>MGSKLINVEGGNNQDDNKYNSNNVISINNKVNKNDYFIETNKELKINLNFQNNNIISNIFSNINIYDKISNIFINNKKTYMLKYNNNINEENFFISYFEKKDDNFVPISPWHHIDLKNDDGTYNMIVEITKYNYIKLEIQLREKFNVIKQDKKKGKLRYYHNSIYWNYGALPQTYEYPKHIYQNKSKKNKEALLFTGDNDPLDILDIGSACLKIGQVVPVKILGAFTLIDEGELDWKIIAINKEDKHYEDINSLSDIEKYYPHTLSLLLEWFRSYKMADTKKLNLISKQLYDKKESEDLIMKTHHYYLEFREDVKKLKEEHSKETIKEHDYVNAQNIQFNYDK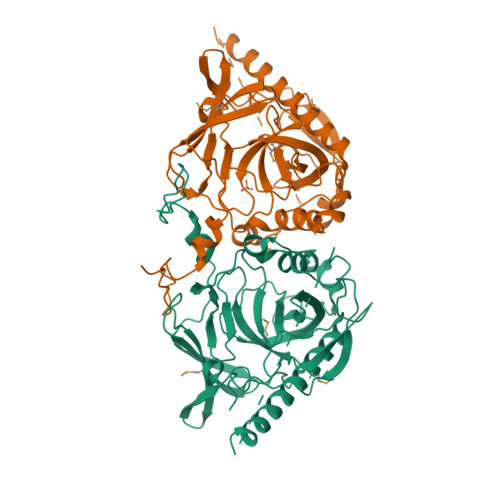LNNNDDEPMENNLLEDINITYYKSDSAYKPDLNIWTP[5x]>MTAALHIGHLSKSFQNTPVLNDISLSLDPGEILFIIGASGCGKTTLLRCLAGFEQPDSGEISLSGKTIFSKNTNLPVRERRLGYLVQEGVLFPHLTVYRNIAYGLGNGKGRTAQERQRIEAMLELTGISELAGRYPHELSGGQQQRAALARALAPDPELILLDEPFSALDEQLRRQIREDMIAALRANGKSAVFVSHDREEALQYADRIAVMKQGRILQTASPHELYRQPADLDAALFIGEGIVFPAALNADGTADCRLGRLPVQSGAPAGTRGTLLIRPEQYSLHPHSAPAASIHAVVLKTTPKARHTEISLRAGQTVLTLNLPSAP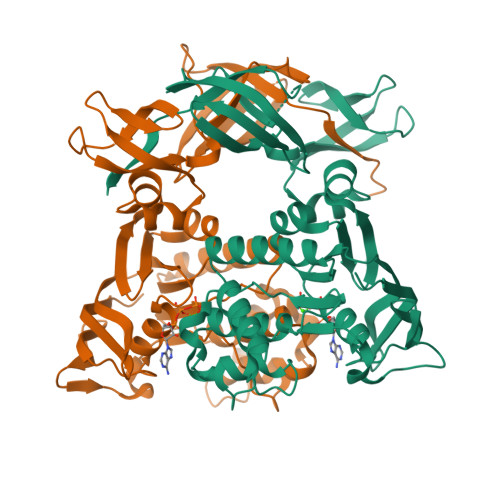TLSDGISAVLHLDGPALFFPGNTLEHHHHHH[2x]(2S)-3-METHYL-2-((2R,3S)-3-[(METHYLSULFONYL)AMINO]-1-{[2-(PYRROLIDIN-1-YLMETHYL)-1,3-OXAZOL-4-YL]CARBONYL}PYRROLIDIN-2-YL)BUTANOIC 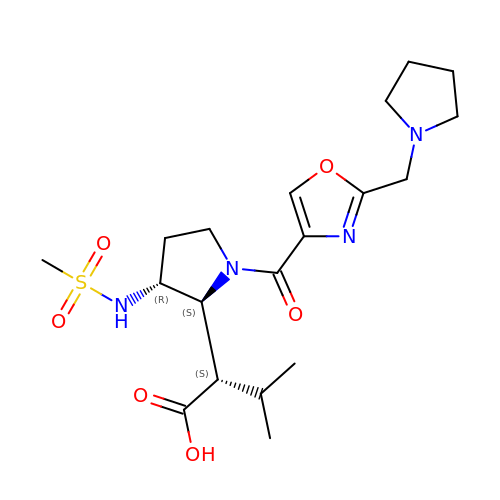ACID | C19 H30 N4 O6 S | PWBJTGRBTWYVSH-XOKHGSTOSA-N> KLKKVLDKLRLKRKDIS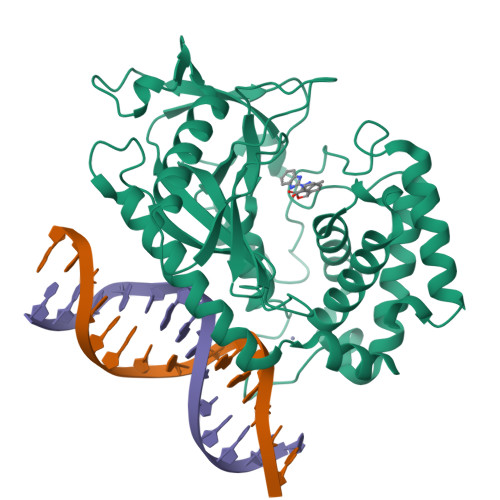EAAETVNKVVERLLRRMQKRESEFKGVEQLNTGSYYEHVKISAPNEFDVMFKLEVPRIELQEYYETGAFYLVKFKRIPRGNPLSHFLEGEVLSATKMLSKFRKIIKEEVKEIKDIDVSVEKEKPGSPAVTLLIRNPEEISVDIILALESKGSWPISTKEGLPIQGWLGTKVRTNLRREPFYLVPKNAKDGNSFQGETWRLSFSHTEKYILNNHGIEKTCCESSGAKCCRKECLKLMKYLLEQLKKEFQELDAFCSYHVKTAIFHMWTQDPQDSQWDPRNLSSCFDKLLAFFLECLRTEKLDHYFIPKFNLFSQELIDRKSKEFLSKKIEYERNNGFPIFD>[2x]MVRGRVPQIQARQINIFGIVQGVGFRPFVFNIAQKYNLKGIVYNNSSGLYIEVEGEEKDIEAFIREIKENPPSLSVIDEIQVREVEVKEYKDFKIVGSKEDGGFVPVSPDMGVCEDCLRELKDPKDRRYRYPFINCTNCGPRFSIIEDIPYDRAKTSMKVFPMCEKCSREYHDPHDRRFHAQPVACFDCGPSLSFVGEGCFDDEIKCVAKALKEGKIVAIKGIGGFHLAVNALDDEAVATLRRRKKRYG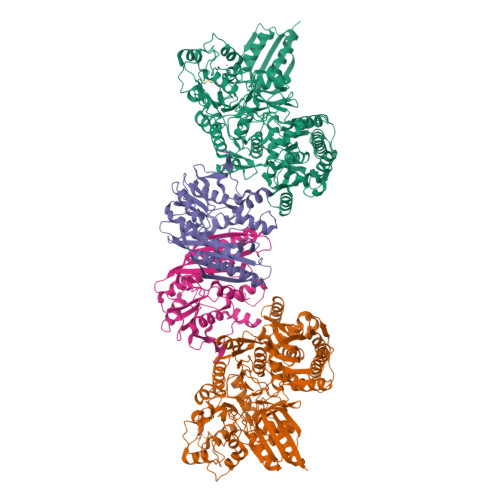KPFAVMMRDVEEVKKYCIVSPEEERLLLSQRRPIVLLKKKGEKLAKGIADDLDTLGVMLPYAPIHYLLMEEIDFPIVMTSGNVSEEPICKDNEEALEKLKDIADVFLLNNRDIVNRIDDSVTSFNAGAERIIRRARGYAPQPILLKKEVKASILAVGGFYKNTFCMTKGHYAFISHHIGDLDNEKAFNYYIEQIERYKKLFRVDPEVVAHDMHKGYLSTQYAKSLDLPKIEVQHHHAHIASCMAEHNLDEKVIGIAYDGTGYGTDGNVWGAEILVCDLKSFERIAHLKYKPLPGNELAIKKIYRTALGFIFDNISFYKNFVEQVDSRELDIILKQIDRKINTAYVSSMGRFFDAVAALIGVRKEVLFEGQAAMELESLMAESEEYYEYEILKEDRYVIDPELILRQIYEDYMKGFEKSYISAKFHNTVVNFTYDLANLIRKETGINKVVLSGGSFQNRYLLRRLIEKLSLSGFEVYSNSKVPCNDGGISLGQAVIANKILEGSAWSHPQFEK;>[2x]GALIEEVFADAFDNEYIRAMEDAALLFGNITLTTDSFTVKPLFFPGGDIGKLAVCGTVNDASMRGAKPLFLTAAFIIEEGFPVEDLKKIVKSMAEAAKEAGVKIVAGDTKVVEKGSVDRIFINTSGIGVLYEGANVSIKNAKPGDIVLISGTIGDHGMAVMSAREELQFDTPIFSDVAPLNGLIEKLMTLGEAIKVLRDPTRGGVAEVLYEISKMSGVGIKIYEEKLPVKESVKSACEFMGIDFLHLANEGKVVVVVERDYAEKALEIMKSHEYGKDAEIIGEVNDSKLVTINTIYGTSRIVDRPIGELLPRIC>[2x]SVKEFQNLVDQHITPFVALSKKLAPEVGNQVEQ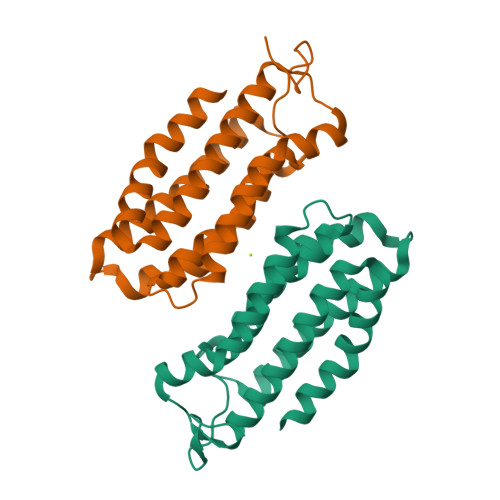LVKAIDAEKALINTASQSKKPSQETLLELIKPLNNFAAEVGKIRDSNRSSKFFNNLSAISESIGFLSWVVVEPTPGPHVAEMRGSAEFYTNRILKEFKGVNQDQVDWVSNYVNFLKDLEKYIKQYHTTGLTWNPKGGDAKSAT>[2x]MRGSHHHHHHGKQLTILGSTGSIGCSTLDVVRHNPEHFRVVALVAGKNVTRMVEQCLEFSPRYAVMDDEASAKLLKTMLQQQGSRTEVLSGQQAACDMAALEDVDQVMAAIVGAAGLLPTLAAIRAGKTILLANKESLVTCGRLFMDAVKQSKAQLLPVDSEHNAIFQSLPQPIQHNLGYADLEQNGVVSILLTGSGGPFRETPLRDLATM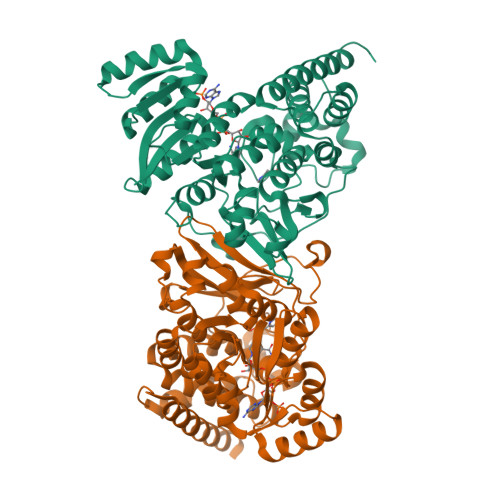TPDQACRHPNWSMGRKISVDSATMMNKGLEYIEARWLFNASASQMEVLIHPQSVIHSMVRYQDGSVLAQLGEPDMRTPIAHTMAWPNRVNSGVKPLDFCKLSALTFAAPDYDRYPCLKLAMEAFEQGQAATTALNAANEITVAAFLAQQIRFTDIAALNLSVLEKMDMREPQCVDDVLSVDANAREVARKEVMRLASSACDLGTPGRPA> GLEDCDFGWSPYDQHCYQAFNEQKTWDEAEKFCRAQENGAHLASIESNGEADFVSWLISQKDELADEDYVWIGLRAQNKE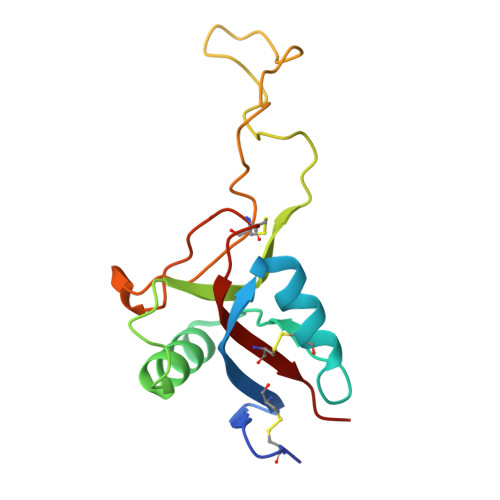QQCSSEWSDGSSVSYENLIDLHTKKCGALEKLTGFRKWVNYYCEQMHAFVCKLLPY> TQQEIFDKQRRLQELSEKVRTCHQEISALRKALQEKEAEMLQVLEDIQT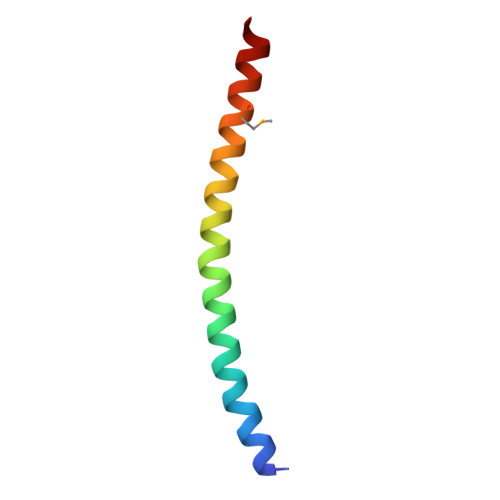I> SMTDTRRRVKVYTLNEDRQWDDRGTGHVSSGYVERLKGMSLLVRAESDGSLLLESKINPNTAYQKQQDTLIVWSEAENYDLALSFQEKAGCDEIWEKICQVQGKD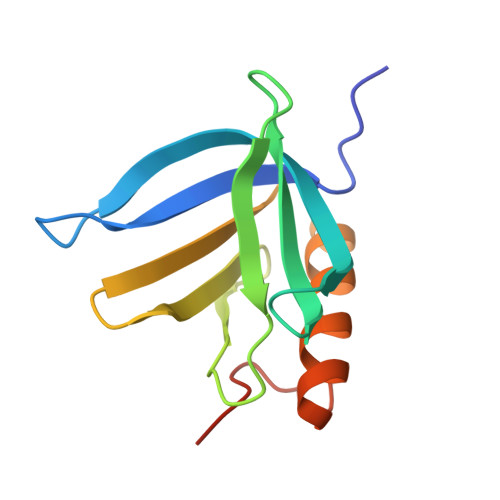PSVDITQDLVDES While this level of potency did not warrant follow-up itself, the hit remained of interest because, simultaneously, 1 was identified in a screen against malarial lysyl-tRNA synthetase (IC50 5 µM). This class of enzyme uses ATP, to ligate the amino acid lysine to its uncharged tRNA, making lysyl-tRNA available for use by the protein synthesis machinery. Genetic analysis has shown that in M. tuberculosis the lysyl-tRNA synthetase gene (lysS) is essential. M. tuberculosis LysRS consists of an N-terminal anticodon binding domain (residues 1–150) with the typical oligonucleotide binding fold, common to lysyl-, asparaginyl- and aspartyl- tRNA synthetases, consisting of a central six-stranded beta-barrel with loops or alpha helices connecting the strands. The C-terminal catalytic domain (residues 151–505) consists of a largely antiparallel beta-sheet flanked by alpha helices, typical of class II aminoacyl-tRNA synthetases.

Initial SAR exploration for the series: exchanging the pyrimidine for a pyridine, expansion of the cyclopentyl to cyclohexyl, and replacement of the H in the 4-position with F were all tolerated and improved potency, although with no selectivity over the human ortholog KARS1. The observed improvement in potency was enough to allow the first compound/protein structures to be obtained, following soaking of ligands into Apo crystals. Structural characterization of ligands showed them to bind in the adenosine pocket, stacked between the side chains of Phe269 and Arg481. In contrast, a small 4-fluoro-substituent, which does not enter the selectivity pocket and had no selectivity at the enzyme level, surprisingly showed an increase in inhibition of the mutant protein compared to the WT. The early, non-selective molecule 2, blocked expression of both COX1 and SDHA, indicating inhibition of both cytoplasmic and mitochondrial translation, whereas treatment with 7, 5, or 8 (≤100 µM) did not inhibit the production of either COX1 or SDHA. The MIC potency for the series was not impacted when performed in the presence of 1 mM lysine, unlike mupirocin (with isoleucine); this was not unexpected, because from the co-crystal structures compound binding did not involve the lysine binding site.

> MGSSHHHHHHSSGENLYFQGHMSAADTAEDLPEQFRIRRDKRARLLAQGRDPYPVAVPRTHTLAEVRAAHPDLPIDTATEDIVGVAGRVIFARNSGKLCFATLQDGDGTQLQVMISLDKVGQAALDAWKADVDLGDIVYVHGAVISSRRGELSVLADCWRIAAKSLRPLPVAHKEMSEESRVRQRYVDLIVRPEARAVARLRIAVVRAIRTALQRRGFLEVETPVLQTLAGGAAARPFATHSNALDIDLYLRIAPELFLKRCIVGGFDKVFELNRVFRNEGADSTHSPEFSMLETYQTYGTYDDSAVVTRELIQEVADEAIGTRQLPLPDGSVYDIDGEWATIQMYPSLSVALGEEITPQTTVDRLRGIADSLGLEKDPAIHDNRGFGHGKLIEELWERTVGKSLSAPTFVKDFPVQTTPLTRQHRSIPGVTEKWDLYLRGIELATGYSELSDPVVQRERFADQARAAAAGDDEAAVLDEDFLAALEYGMPPCTGTGMGIDRLLMSLTGLSIRETVLFPIVRPHSN DIGUANOSINE-5'-TRIPHOSPHATE | C20 H27 N10 O18 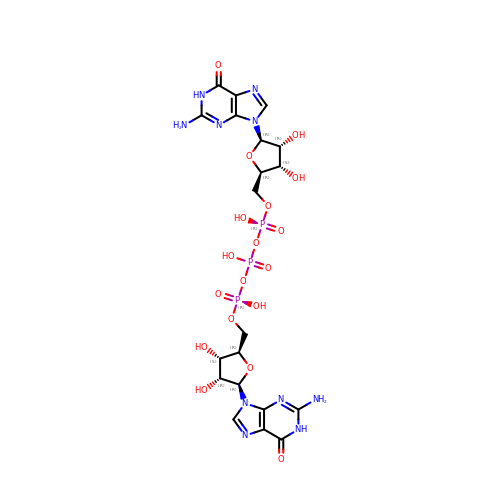P3 | AAXYAFFKOSNMEB-MHARETSRSA-N>ELFRGVLQVSSNVLDCANDNWWCSLLDLDTSDWEPLTHTNRLMAIYLSSVASKLDFTGGPLAGCLYFFQVECNKFEEGYHIHVVIGGPGLNPRNLTVCVEGLFNNVLYHLVTGNVKLKFLPGMTTKGKYFRDGEQFIENYLMKKIPLNVVWCVTNIDGYIDTCISATFRRGACHAKKPRMTTAINDTSSDAGEPSGTGAEVVPFNGKGTKASIKFQTMVNWLCENRVFTEDKWKLVDFNQYTLLSSSHSGSFQIQSALKLAIYKATNLVPTSTFLLHADFEQVMCIKDNKIVKLLLCQNYDPLLVGQHVLKWIDKKCGKKNTLWFYGPPSTGKTNLAMAIAKSVPVYGMVNWNNENFPFNDVAGKSLVVWDEGIIKSTIVEAAKAILGGQPTRVDQKMRGSVAVPGVPVVITSNGDITFVVSGNTTTTVHAKALKERMVKLNFTVRCSPDMGLLTEADVQQWLTWCNAQSWDHYENWAINYTFDFPGINADALHPDLQTTPIVTDTSISSSGGESSEELSESSFFNLITPGACNTETPRSSTPIPGTSSGESLVGSPVSSEVVAASWEE[12x]

The main replication protein NS1 plays a critical role in cell cycle arrest, transactivation of viral and host genes, and replication and package of B19V genome. Based on its similarity to other parvoviral replication proteins, such as Rep72 of the adeno-associated virus (AAV), NS1 is predicted to contain one nuclease domain (Nuc, aa 1–176), one oligomerization domain (OD, aa 201–270), one SF3 helicase domain (SF3 HD, aa 271–501), and one zinc-binding domain (ZnD, aa 571–671). The SF3 HD domain of NS1 belongs to the SF3 helicase superfamily, which unwinds DNA with 3′→5′ polarity. Totally, four cryo-electron microscopy (cryo-EM) structures were determined, which revealed the detailed mechanisms for ATP binding and hydrolysis and DNA binding and unwinding by NS1.

To reveal how NS1 recognizes DNA duplex, we performed further cryo-EM study using fork DNA-2 and solved one NS1_2-570/dsDNA/AMPPNP ternary complex at an overall resolution of 3.43 Å. Like the NS1_2-570/AMPPNP structure, NS1 forms dodecamer in the dsDNA-bound structure. As supported by the low RMSD value (0.8 Å), dsDNA binding does not cause significant change to the conformation and overall assembly of NS1 in the dsDNA-bound structure. The density maps suggested that dsDNA could be bound by both NS1 hexamers, hexamer-1 and hexamer-2. However, due to the density associated with hexamer-2 is relatively weak, only the DNA bound by hexamer-1 is modeled in the final structure. The DNA adopts regular B-form-like conformation; it is inclined toward one side of the ring formed by the OD domains. The side chains of Thr210 of NS1 protomers A, E, and F point toward the DNA, forming H-bond interactions with the backbone phosphate groups of +6, +2, and +4 nucleotides, respectively. Instead of interacting with the phosphate group, the side chain of Lys211 points toward the major groove of the DNA. In the dsDNA-bound NS1 structure, the side chain of the His249 wraps around the DNA backbone from the major or minor groove sides. The 3′-end nucleotide of the DNA is inserted into the central ring formed by the OD domains, further confirmed the 3′→5′ unwinding polarity of NS1.>[2x]MDVSYLLDSLNDKQREAVAAPRSNLLVLAGAGSGKTRVLVH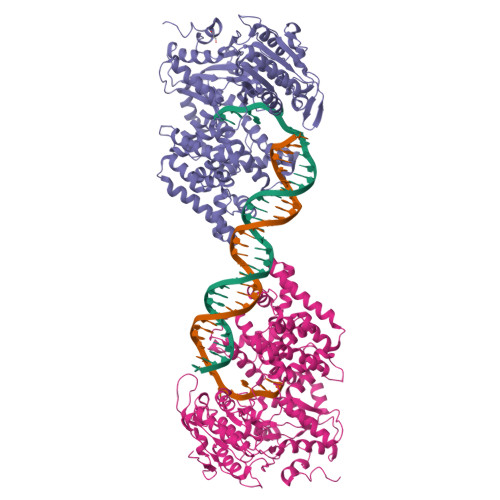RIAWLMSVENCSPYSIMAVTFTNKAAAEMRHRIGQLMGTSQGGMWVGTFHGLAHRLLRAHHMDANLPQDFQILDSEDQLRLLKRLIKAMNLDEKQWPPRQAMWYINSQKDEGLRPHHIQSYGNPVEQTWQKVYQAYQEACDRAGLVDFAELLLRAHELWLNKPHILQHYRERFTNILVDEFQDTNNIQYAWIRLLAGDTGKVMIVGDDDQSIYGWRGAQVENIQRFLNDFPGAETIRLEQNYRSTSNILSAANALIENNNGRLGKKLWTDGADGEPISLYCAFNELDEARFVVNRIKTWQDNGGALAECAILYRSNAQSRVLEEALLQASMPYRIYGGMRFFERQEIKDALSYLRLIVNRNDDAAFERVVNTPTRGIGDRTLDVVRQTSRDRQLTLWQACRELLQEKALAGRAASALQRFMELIDALAQETADMPLHVQTDRVIKDSGLRTMYEQEKGEKGQTRIENLEELVTATRQFSYNEEDEDLMPLQAFLSHAALEAGEGQADTWQDAVQLMTLHSAKGLEFPQVFIVGMEEGMFPSQMSLDEGGRLEEERRLAYVGVTRAMQKLTLTYAETRRLYGKEVYHRPSRFIGELPEECVEEVRLRATVSRPVSHQRMGTPMVENDSGYKLGQRVRHAK>[2x]MGGSHHHHHHRSESTVTEELKEGIDAVYPSLVGTADSKAEGIKNYFK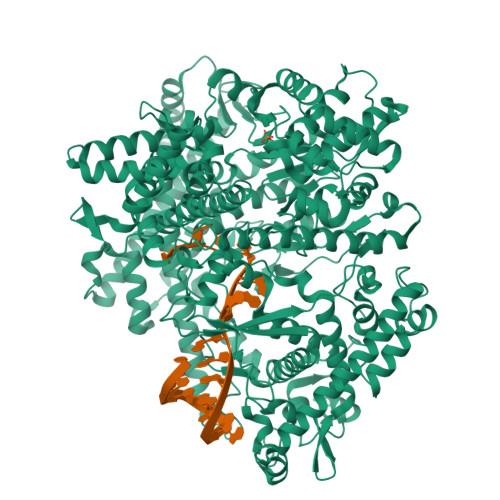LSFTLPEEQKSRTVGSEAPLKDVAQALSSRARYELFTEKETANPAFNGEVIKRYKELMEHGEGIADILRSRLAKFLNTKDVGKRFAQGTEANRWVGGKLLNIVEQDGDTFKYNEQLLQTAVLAGLQWRLTATSNTAIKDAKDVAAITGIDQALLPEGLVEQFDTGMTLTEAVSSLAQKIESYWGLSRNPNAPLGYTKGIPTAMAAEILAAFVESTDVVENIVDMSEIDPDNKKTIGLYTITELDSFDPINSFPTAIEEAVLVNPTEKMFFGDDIPPVANTQLRNPAVRNTPEQKAALKAEQATEFYVHTPMVQFYETLGKDRILELMGAGTLNKELLNDNHAKSLEGKNRSVEDSYNQLFSVIEQVRAQSEDISTVPIHYAYNMTRVGRMQMLGKYNPQSAKLVREAILPTKATLDLSNQNNEDFSAFQLGLAQALDIKVHTMTREVMSDELTKLLEGNLKPAIDMMVEFNTTGSLPENAVDVLNTALGDRKSFVALMALMEYSRYLVAEDKSAFVTPLYVEADGVTNGPINAMMLMTGGLFTPDWIRNIAKGGLFIGSPNKTMNEHRSTADNNDLYQASTNALMESLGKLRSNYASNMPIQSQIDSLLSLMDLFLPDINLGENGALELKRGIAKNPLTITIYGSGARGIAGKLVSSVTDAIYERMSDVLKARAKDPNISAAMAMFGKQAASEAHAEELLARFLKDMETLTSTVPVKRKGVLELQSTGTGAKGKINPKTYTIKGEQLKALQENMLHFFVEPLRNGITQTVGESLVYSTEQLQKATQIQSVVLEDMFKQRVQEKLAEKAKDPTWKKGDFLTQKELNDIQASLNNLAPMIETGSQTFYIAGSENAEVANQVLATNLDDRMRVPMSIYAPAQAGVAGIPFMTIGTGDGMMMQTLSTMKGAPKNTLKIFDGMNIGLNDITDASRKANEAVYTSWQGNPIKNVYESYAKFMKNVDFSKLSPEALEAIGKSALEYDQRENATVDDIANAASLIERNLRNIALGVDIRHKVLDKVNLSIDQMAAVGAPYQNNGKIDLSNMTPEQQADELNKLFREELEARKQKVAKAR> MAAQVLSGHEAAEAVYEEIRARLRSLSFTPSLRVIRLGEDPASVAYVRLKDKRARALGYRSQVEVYPEDLPEEALLERIAALNADEEVDGILVQLPLPPHIRTQRVLEAIHPLKDVDGFHPLNVGRLWSGGKGLFPCTPLGVVRLLKHYGVDLRGKEVVVVGRSNIVGKPLAGLLLREDATVTLAHSKTQDLPEVTRRAQVLVVAVGRPHLVRKEWVREGAIVVDVGVNRVEGRLLGDVHPEVAEVAFALTPVPGGVGPMTVAMLM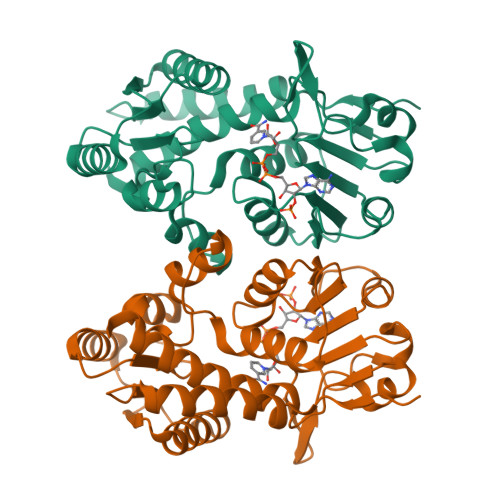GNTLEAALLRR>SNAMGMINVFQPTLGEAELAAVREVFASGWLGRGPRTKVFEADFAEHLGVGAEQVVSVSCCTEGLFLSMELLGVGPGDEVVLPSISFVGAANAIAARGARPVFCDVDPATLNPTADHVAEKLGPRTKAVVVLHYGGYPGDLVAI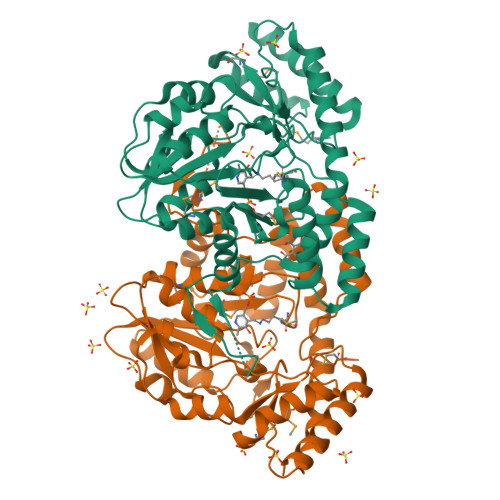AELCRERGVPLVEDSACAVASQVDGRACGTLGDVGVWSFDAMKILVTGDGGMLCFRDPELAERARKLASLGMAQSSGFANATADAEARWWEFEVTAFGRRSISNDVAASIGSVQLRRLPEFVRRRREIAERYDQGLSTVDGLRCPPPLPAGHTSSYYFYWVRMDASVRDAMARRLYDRGVYTTFRYAPLHLVSAYGHEGSLPGAERAAEETLCLPLHQALSDSDVETVIGEVRAGLAALTAPSGSSVPTVSSFPASRP[4x]>[40x]MSVVTKSIVNADAEARYLSPGELDRIKNFVSTGERRLRIAQTLTENRERIVKQAGDQLFQKRPDVVSPGGNAYGEEMTATCLRDLDYYLRLVTYGIVAGDVTPIEEIGLVGVREMYNSLGTPIPAVAEGIRAMKNVACSLLSAEDAAEAGSYFDFVIGAMQ;>MQDAITAVINASDVQGKYLDTAAMEKLKAYFATGELRVRAASVISANAANIVKEAVAKSLLYSDITRPGGNMYTTRRYAACIRDLDYYLRYATYAMLAGDPSILDERVLNGLKETY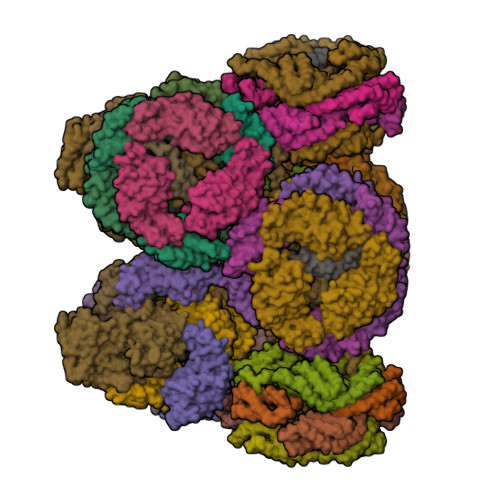NSLGVPIAATVQAIQAMKEVTASLVGADAGKEMGIYFDYICSGLS[40x];>MVVKASGGSSVARPQLYQTVPVSTIIQAEQQDRFLNRGELDELAVYLRSGAKRLEIATTLTRNADIIVSRAANRIFVGGSPMAFLSRPQTEEAPQFTTGARGEAIDIKEAMKLGTATYVDTRGGFLEGLRSIFSASSGGAPVGFKPINIARYGPARMEKSLRDLDWFLRYTTYAIVAGDPNILAVNTRGLREIIEAACSSDATIAALQEMRRAALSYFEKDAEAKGIVETYFDVLINEFIAPAPSDKVRQRNSTDLQGLQLPQIYFNAAERRPKFVMKPGLSAAEKNEVVKAAYRQIFERDISRAYGLGISDLESKVKNGSISMKEFIRQLAKSPLYRKNFYEPYINSRALELAFRHILGRGPSSREEVQTYFAIISKGGLPALVDALVDSKEYSDYFGEETVPYLRGLGQEAQECRNWGAQQDLFKYSAPFRKVPQFITTFAAQDQPLPDQHPYGSGNDPLEIQFGAIFPKEKKNPSARPQPFNKDTRRILIARGPGINNQVSNPGARGLTPGTLGPKVFKLDQLPSINARIGKRSIATGTDSVKFAESSTQRVIRAAYLQVFGRDVYEGQRQKVAEIKLENGEISVREFVRILAKSNLFRSLYWTPLYVTKAIEYIHRRLLGRPTYGRQEMNAYFDIASKKGLYGLVDAIIDSQEYSEAFGEDTVPYERYITPQGLALRSLRVGTIGETGVPPEKEETPRFVELGAVTELRTEPAIQFRANQGVSKRREQTKVFKLTDLNDKQNLQLVIQAAYRQVFERDVAPYIVRDEFTALESKLSNGEITLKEFIEALGCSELYQKEFYTPYPNTKVIELGTKHFLGRAPLDQAEIRRYNQILATQGLKAFVQALVSSAEYAQAFGEDTVPYRRFPTLPAANFPNTEKLHNQLTKQSDAIVVPSFAPVKPRLDNTKLPLLSRAIAEQEAKARQADPSKPRFIELGRSFRNGDGQSVEVGVGTTRRRPARIFRMTVGAPSAEVELVINAIYCQVMDVFSGQVPSQFRRPDLESRLRNGEITVREFVRTLASSEIYRNRFYTPYPNTKVIEFLFRHLLGRAPATQAEIRQYNKILADQGLKTAVETMVNSPEYSRYFGEDVVPYKRFPTLPAGNYIGSVKADADLVKQSWSSLSPSLVGIQPSHRD[2x];>[2x]MRDAVTTLIKNYDSTGRYLDRDAVDRLRSYFNSGAARVKAAAVINANAAAIVKEAASALFTEQPELIQPGGNAYTTRRYATCLRDMDYYLRYASYAIVAGDVDVLNERVLEGLRETYNSLGVPIGPTVRGIQIMKEIVRDRVAAAGIEDTGIVEQPFDYMCRQLSEVNI;>[6x]MRMFKITACVPSQTRIRTQRELQNTYFTKLVPYENWFREQQRIQKMGGKIVKVELFTGKPGVNTGLA>[6x]GSADLIKKKLPFR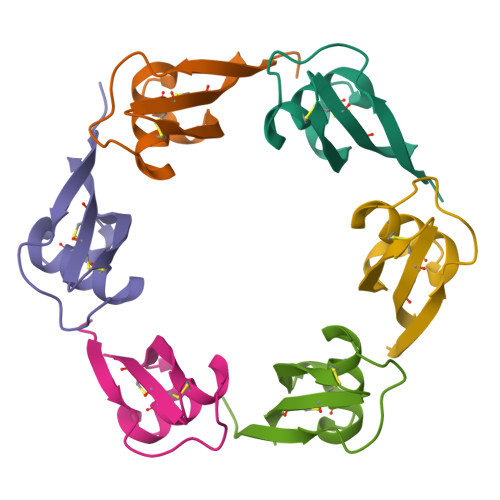TRSKFPRKSECVQDCAKAFTNGNKDKIKDVKSEFFSCYCWYEA>[2x]MGSSHHHHHHSSGENLYFQGHMESALAVPRLPPHDPGTPVLSVVDMHTGGEPLRIVLAGCPEVSGPTLLAKRRYMRQHLDHVRRRLMFEPRGHRDMYGAVLVPSELPDAHLGVLFLHNEGYSSMCGHAVLALGRFALDFGLVPAP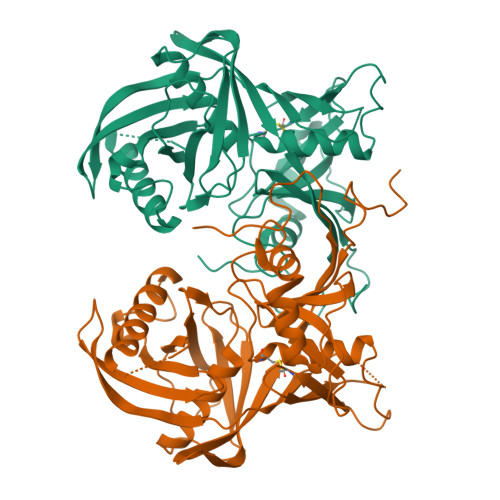PAGTREARVNIHCPCGLVTAFVACEDGRSHGPVRFHSVPAFVLATDLMVDVPGHGKVMVDIAYGGAFYAFVTAEKLGLDICSAKTRDLVDAASAVTEAVKAQFKINHPDSEDLAFLYGTILTDGKDAYTKEPTTNICVFADEQVDRSPTGSGVTARIALQYHKGLLELNQMRAFKSSATGSVFTGKAVREAKCGDFKAVIVEVSGQAHYTGTASFIIEDDDPLRDGFLLK High-resolution crystal structures and biophysical analyses of a truncated form of the TbMORN1 protein and its homologues from the parasites Toxoplasma gondii (TgMORN1) and Plasmodium falciparum (PfMORN1) enabled, for the first time, a structure-based definition of the MORN repeat. All three structures are antiparallel dimers joined via their C-termini, and, when possessed of the correct key residues, can adopt extended or V-shaped quaternary structures. The crystal structures confirmed that each 23-amino acid MORN repeat is composed of a β-hairpin followed by a 6-residue loop that connects to the next MORN repeat. The structural studies presented here make a case that one conserved function of MORN repeats is in homotypic interactions and possibly also in higher-order assembly.

Although TgMORN1(7–15) was predominantly found as an extended dimer, a V-shaped form similar to that of PfMORN1(7–15) was also observed in the crystal lattice. The two V-shaped dimers share the same coordination sphere of a Zn2+ ion, which in TgMORN1(7–15) is provided by the Cys305 and Asp308 residues. The latter residue in turn interacts with the Ser310 from the other subunit. While the salt bridge and anion π-interactions are also conserved between the two V-shaped dimers, the aromatic stacking present in the core of the PfMORN1(7–15) dimer interface is functionally replaced in the TgMORN1(7–15) V-shaped dimer by a series of aromatic stacking interactions at its vertex. The coordination residues map to the β-hairpin of MORN repeat 13, which in TgMORN1 and PfMORN1, but not TbMORN1, contains an insertion of a glutamate residue—Glu307 and Glu308, respectively. Taking part in an anion π-interaction with a phenylalanine residue (Phe303 and Phe304, respectively), the resulting Glu-Phe pairs effectively stabilise the TgMORN1 and PfMORN1 dimers in their V-shaped form. Moreover, these very same glutamate residues further stabilise the two V-shaped dimers by being involved in a salt bridge with lysine residues (Lys321 in TgMORN1 and Lys322 in PfMORN1). The residues in the crystal structures of TgMORN1(7–15) and PfMORN1(7–15) forming the Zn2+-coordination sphere and anion π-interaction were taken as a fingerprint for a V-shaped dimer. Based on the crystallographic data, the apicomplexan MORN1 proteins appear capable of forming both extended and V-shaped conformations. MORN1 proteins in Apicomplexa have been shown to be a key component of the basal complex, which undergoes a constriction event at the end of the cell division cycle. It is therefore tempting to speculate that these extended (Zn-free) and V-shaped (Zn-bound) conformations represent the pre- and post-constriction states of the MORN1 proteins in the basal complex.

> EKYEGDWVNGKMHGHGKYIYSDGGVYEGDWIDGKMHGKGTYVFPNGNVYEGEWAHDMKDGYGVLTYQNGEKYEGYWKQDKVHGKGTLTYTRGDKYIGDWMDAKKDGEGELIYANGDRFKGQWADDRANGFGVFTYANGNRYEGEWTDDKRHGRGVFYCAEDGSAYEGEFVGGRKEGNGILRLATGHQLEGTWSGGQLVRVTSFVFAQDSPWLNVDL> TDDSEK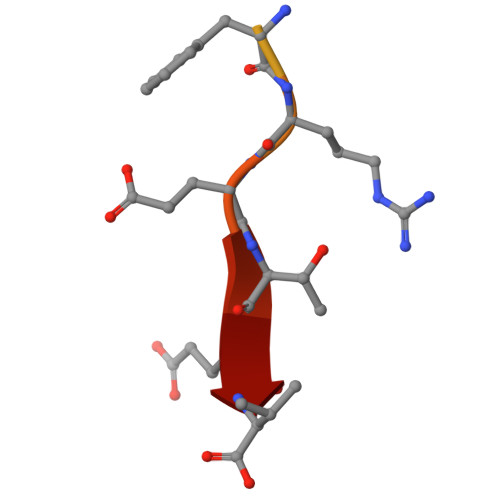HFRETEV> VTSYTLNEVVPLKDVV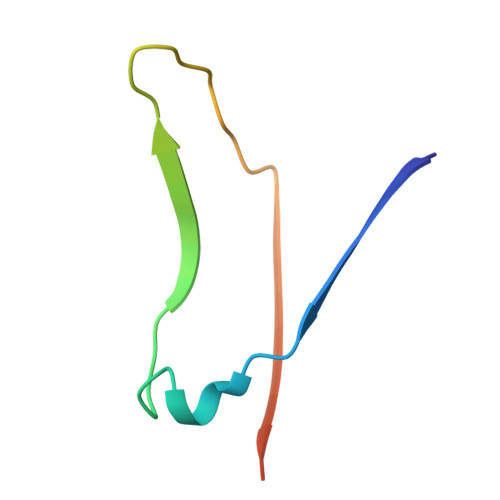PEWVRIGFSATTGAEFAAQEVHSWSFNSQLGHTSKS>[2x]MKVQYCDSLVIGGGLAGLRAAVATQQKGLSTIVLSLIPVKRSHSAAAQGGMQASLGNSKMSDGDNEDLHFMDTVKGSDWGCDQKVARMFVNTAPKAIRELAAWGVPWTRIHKGDRMAIINAQKTTITEEDFRHGLIHSRDFGGTKKWRTCYTADATGHTMLFAVANECLKLGVSIQDRKEAIALIHQDGKCYGAVVRDLVTGDIIAYVAKGTLIATGGYGRIYKNTTNAVVCEGTGTAIALETGIAQLGNMEAVQFHPTPLFPSGILLTEGCRGDGGILRDVDGHRFMPDYEPEKKELASRDVVSRRMIEHIRKGKGVQSPYGQHLWLDISILGRKHIETNLRDVQEICEYFAGIDPAEKWAPVLPMQHYSMGGIRTDYRGEAKLKGLFSAGEAACWDMHGFNRLGGNSVSEAVVAGMIVGEYFAEHCANTQVDLETKTLEKFVKGQEAYMKSLVESKGTEDVFKIKNRMKDVMDDNVGIFRDGPHLEKAVKELEELYKKSKNVGIKNKRLHANPELEEAYRVPMMLKVALCVAKGALDRTESRGAHNREDYPKRDDINWLNRTLASWPNPEQTLPTLEYEALDVNEMEIAPGYRGYGAKGNYIENPLSVKRQEEIDKIQSELEAAGKDRHAIQEALMPYELPAKYKARNERLGDKQRRR;>MGRMLTIRVFKYDPQSAVSKPHFQEYKIEEAPSMTIFIVLNM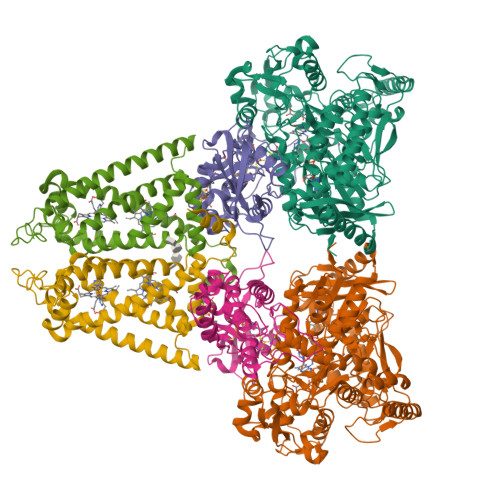IRETYDPDLNFDFVCRAGICGSCGMMINGRPSLACRTLTKDFEDGVITLLPLPAFKLIKDLSVDTGNWFNGMSQRVESWIHAQKEHDISKLEERIEPEVAQEVFELDRCIECGCCIAACGTKIMREDFVGAAGLNRVVRFMIDPHDERTDEDYYELIGDDDGVFGCMTLLACHDVCPKNLPLQSKIAYLRRKMVSVNMS[2x];>MTNESILESYSGVTPERKKSRMPAKLDWWQSATGLFLGLFMIGHMFFVSTILLGDNVMLWVTKKFELDFIFEGGKPIVVSFLAAFVFAVFIAHAFLAMRKFPINYRQYLTFKTHKDLMRHGDTTLWWIQAMTGFAMFFLGSVHLYIMMTQPQTIGPVSSSFRMVSEWMWPLYLVLLFAVELHGSVGLYRLAVKWGWFDGETPDKTRANLKKLKTLMSAFLIVLGLLTFGAYVKKGLEQTDPNIDYKYFDYKRTHEE[2x]> GNGCHANNDTIKVLAIGNSFSQDAVEQYLHELGEAEGITMIIGNMFIGGCSLERHVQNIRNNAPAYAYRKVEKDGEKTETRSMTIEKALADEKWDYISVQQASPLSGIYDSYKASLPELVNYIRERIGKETVLMMHQTWAYATNANHTGFKNYDQNQMKMYTSIVDAVKKAANLVGIKKIIPSGTAIQNARTSFIGDHMNRDGYHLDLTIGRYTAACTWFEALTHRNVTENPYSPEGIDPIH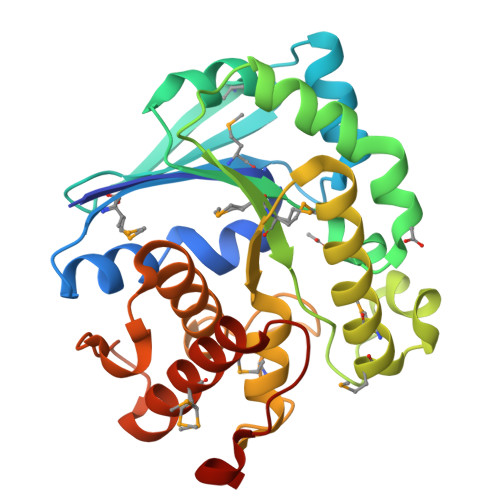KKAAQMAAHNAILYPDKVTELTELKKIAD>MEMEQEKMTMNKELSPDAAAYCCSACHGDETWSYNHPIRGRAKSRSLSASPALGSTKEFRRTRSLHGPCPVTTFGPKACVLQNPQTIMHIQDPASQRLTWNKSPKSVLVIKKMRDASLLQPFKELCTHLMEENMIVYVEKKVLEDPAIASDESFGAVKKKFCTFREDYDDISNQIDFIICLGGDGTLLYASSLFQGSVPPVMAFHLGSLGFLTPFSFENFQSQVTQVIEGNAAVVLRSRLKVRVVKELRGKKTAVHNGLGENGSQAAGLDMDVGKQAM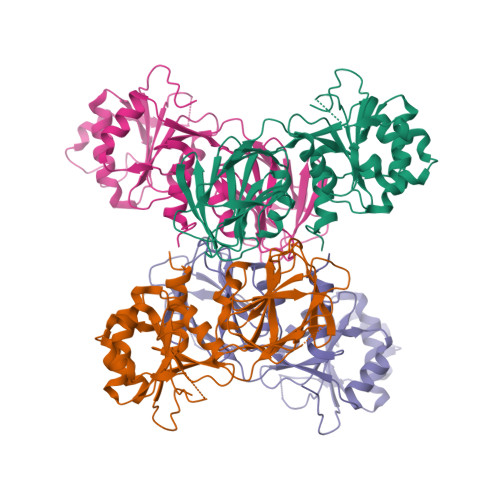QYQVLNEVVIDRGPSSYLSNVDVYLDGHLITTVQGDGVIVSTPTGSTAYAAAAGASMIHPNVPAIMITPICPHSLSFRPIVVPAGVELKIMLSPEARNTAWVSFDGRKRQEIRHGDSISITTSCYPLPSICVRDPVSDWFESLAQCLHWNVRKKQAHFEEEEEEEEEGTRTRPLEQKLISEEDLAANDILDYKDDDDKV[4x]7-aminocephalosporanic acid 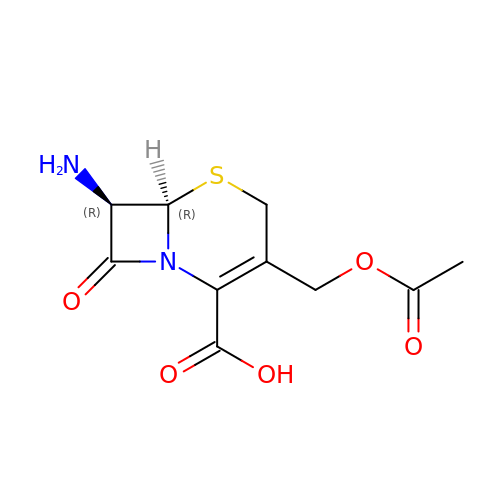| C10 H12 N2 O5 S | HSHGZXNAXBPPDL-HZGVNTEJSA-N>MKNLSAYEVYESPKTSGESRTEAVSEAAFESDPEVSAILVLTSSEASTLERVADLVTAHALYAAHDFCAQAQLAAAELPSRVVARLQEFAWGDMNEGHLLIKGLPQVRSLPPTPTSNVHAVAATTPMSRYQALINECVGRMIAYEAEGHGHTFQDMVPSAMSAHSQTSLGSAVELELHTEQAFSPLRPDFVSLACLRGDPRALTYLFSARQLVATLTTQEIAMLREPMWTTTVDESFLAEGRTFLLGFERGPIPILSGADDDPFIVFDQ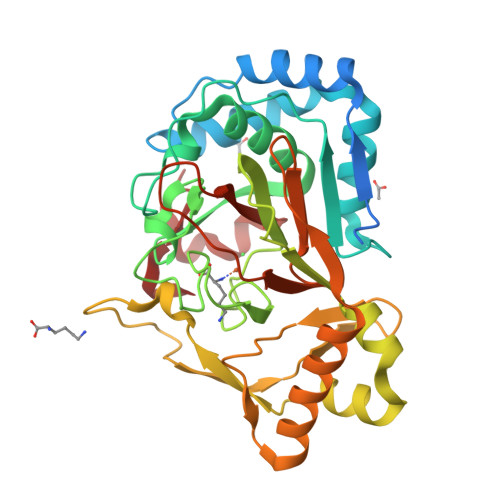DLMRGISAPAQELQQTVIRAYYAERVSHCLAPGEMLLIDNRRAVHGRSIFAPRFDGADRFLSRSFIVADGSRSRHARSSFGRVVSARFS[4x]> MPFTVVTLKSVPPSLRGDLTKWMQEIAIGVYVGNFNSRIREKLWN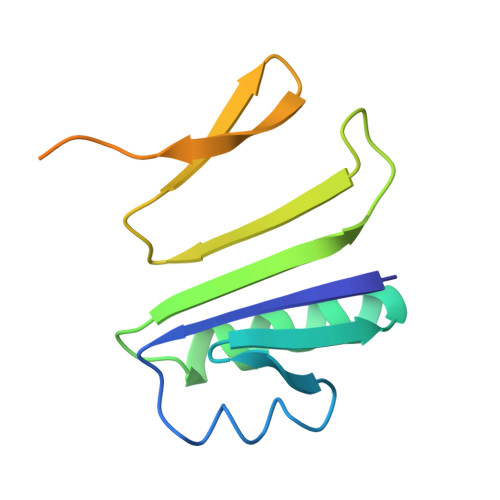RIQANVGEGEATISYYYRNEIGYQFDMINSQKSVVDFDGIPLVLIPNSKTSSENYPKLGYSNAAKSRKIKRYSSYRG>SGRGEAETRECIYYNANWELERTNQSGLERCEGEQDKRLHCYASWRNSSGTIELVKKGCWLDDFNCYDRQECVATEENPQVYFCCCEGNFCNERFTHLPEPLVPR[2x];>[2x]GLECDGKVNICCKKQFFVSFKDIGWNDWIIAPSGYHANYCEGECPSHIAGTSGSSLSFHSTVINHYRMRGHSPFANL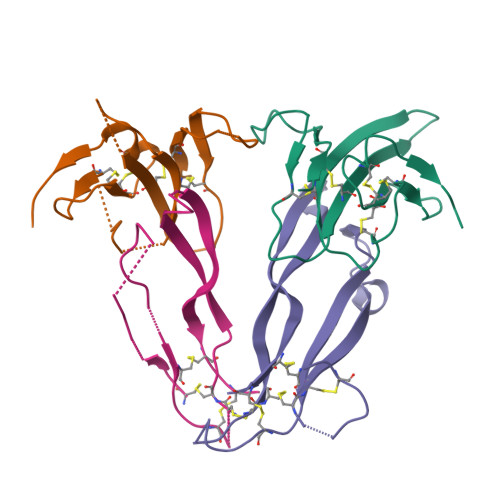KSCCVPTKLRPMSMLYYDDGQNIIKKDIQNMIVEECGCS> PIFLNVLEAIEPGVVCAGHDNNQPDSFAALLSSLNELGERQLV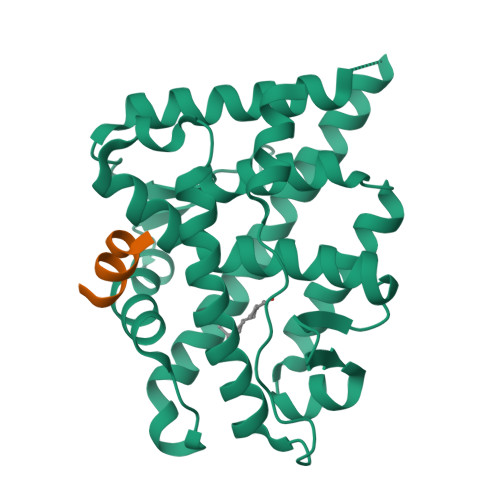HVVKWAKALPGFRNLHVDDQMAVIQYSWMGLMVFAMGWRSFTNVNSRMLYFAPDLVFNEYRMHKSRMYSQCVRMRHLSQEFGWLQITPQEFLCMKALLLFSIIPVDGLKNQKFFDELRMNYIKELDRIIACKRKNPTSCSRRFYQLTKLLDSVQPIARELHQFTFDLLIKSHMVSVDFPEMMAEIISVQVPKILSGKVKPIYFHTQ;> RGAFQNLFQSV2-(2-BENZOFURANYL)-2-IMIDAZOLINE | C11 H8 N2 O | 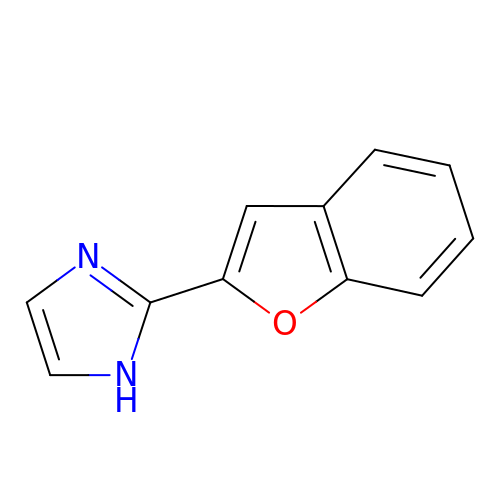VBFQIUOSXHUWCT-UHFFFAOYSA-N>CGUACG[4x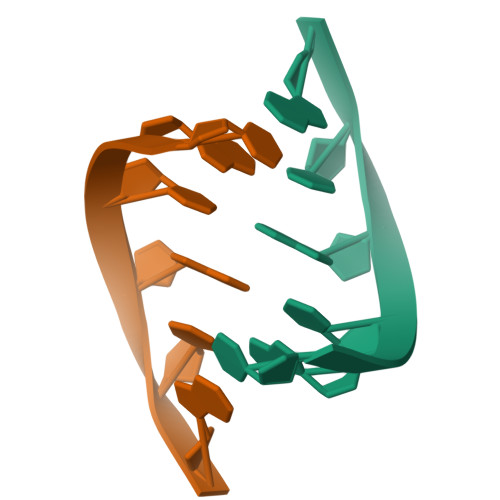]(2R)-4-[(6-CHLORO-2-NAPHTHALENYL)SULFONYL]-6-OXO-1-[[1-(4-PYRIDINYL)-4-PIPERIDINYL]METHYL]-2-PIPERAZINECARBOXYLIC 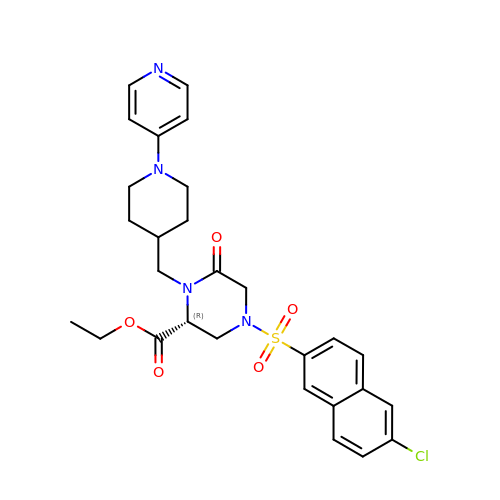ACID ETHYL ESTER | C28 H31 Cl N4 O5 S | BVVKZWAFUVRXPJ-AREMUKBSSA-N> GSKPMEVYVSAVASPTKFWVQLIGPQSKKLASMVQEMTSYYSSAENRAKHV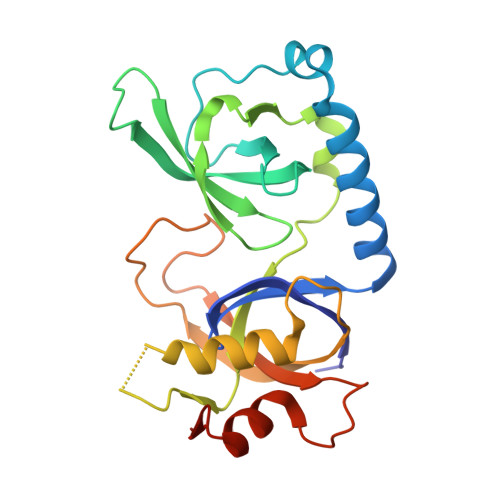LTAPYVGQIVAAVFKFDEKWYRAEIVDIMPNQYNPKEQVIDLYFVDYGDSEYISPADICELRTDFLTLRFQAVECFLANVKSTIQTEPITWPKSSIAKFEELTEVAHWRKLIARVVTYKERPRATTAVSAAAKEGTPLPGVELFDPADNSELNIADLMITQGFALPLDDSYP Here, a microfluidic device is described that enables the production of crystals by counter-diffusion and their direct on-chip analysis by serial crystallography at room temperature. Furthermore, the crystal structures of four proteins and an RNA were determined based on serial data collected on four synchrotron beamlines, demonstrating the general applicability of this multipurpose chip concept.

Final crystal structures were obtained either from a single large crystal and two wedges (Nb02) or from combining partial data sets from several individual crystals (RNA, CCA, Lip and PhP1). In the latter case, the use of ccCluster considerably facilitated the choice of partial data sets to be merged. The analysis in shutterless mode also limits systematic errors in crystal orientation and thus improves the data quality. For example, the highest apparent mosaicity of the RNA crystals, which were analyzed at an early stage of this work with a MAR CCD detector, is a direct symptom of the data-collection strategies used before the advent of HPDs. More generally, the number of crystals that are required for structure determination will depend on their size, their symmetry and their sensitivity to radiation damage. Most of our structures were derived from rather small series of 6–14 crystals and the combination of best data sets.

>CGUGAUCGC[2x]>[6x]SMGARASVLSGGELD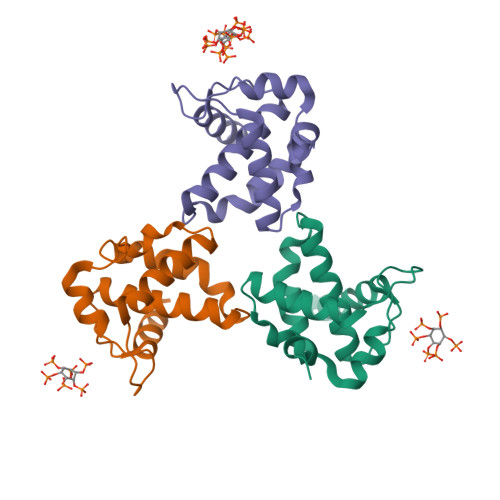KWEKIRLRPGGKKQYKLKHIVWASRELERFAVNPGLLETSEGCRQILGQLQPSLQTGSEELRSLYNTIAVLYCVHQRIDVKDTKEALDKIEEEQNKSKKKAQ> EFPYYLRSFLVVLKTVLENEDDMLLFDEQEKGIVTKFYQLSATGQKLYVRLFQRKLSWIKMTKLEYEEIALDLTPVIEELTNAGFLQTESELQELSEVLELLSAPELKSLAKTFHLVNPNGQKQQLVDAFLKLAKQRSVCTWGKNKPGIGAVILKRAKALAGQSVRICKGPRAVFSRILLLFSLTDSMEDEDAACGGQGQLSTVLLVNLGRMEFPSYTINRKTHIFQDRDDLIRYAAATHMLSDISSAMANGNWEEAKELAQCAKRDWNRLKNHPSLRCHEDLPLFLRCFTVGWIYTRILSRFVEILQRLHMYEEAVRELESLLSQRIYCPDSRGRWWDRLALNLHQHLKRLEPTIKCITEGLADPEVRTGHRLSLYQRAVRLRESPSCKKFKHLFQQLPEMAVQDVKHVTITGRLCPQRGMCKSVFVMEAGEAADPTTVLCSVEELALAHYRRSGFDQGIHGEGSTFSTLYGLLLWDIIFMDGIPDVFRNACQAFPLDLCTDSFFTSRRPALEARLQLIH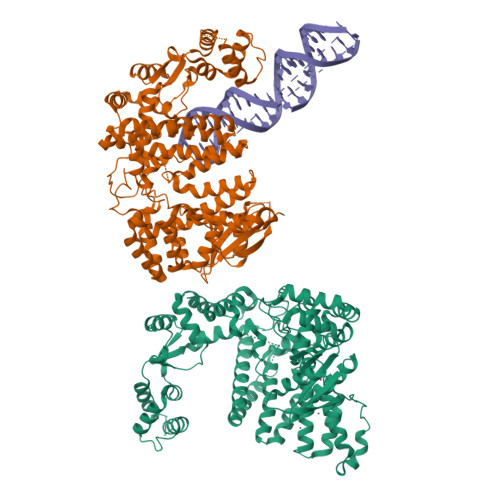DAPEESLRAWVAATWHEQEGRVASLVSWDRFTSLQQAQDLVSCLGGPVLSGVCRHLAADFRHCRGGLPALVVWNSQSRHFKLVEVKGPNDRLSHKQMIWLAELQKLGAEVEVCHVVAVGAKSQSLS> SQDLLDL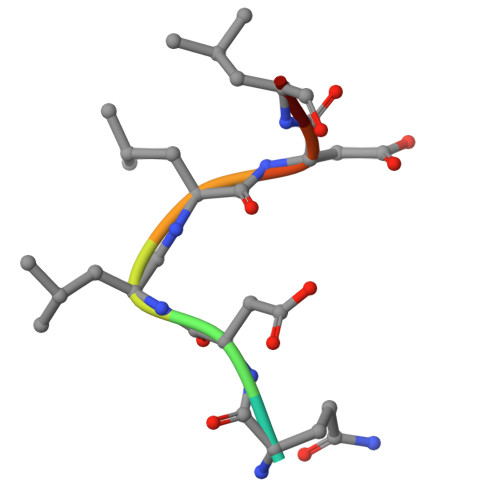F>[2x]MLEKVETFDMNRVIDEFDEMTRNAHQVQKQTLKEILLKNQSAIYLQNCGLNGNATDPEEAFKSMVPLVTDVELEPYIKRMVDGDTSPILTGHPVPAISLSSGTSQGRPKFIPFTDELMENTLQLFRTAFAFRNRDFPIDDNGKALQFIFSSKQYISTGGVPVGTATTNVYRNPNFKAGMKSITSPSCSPDEVIFSPDVHQALYCHLLSGILFRDQVQYVFAVFAHGLVHAFRTFEQVWEEIVTDIKDGVLSNRITVPSVRTAMSKLLTPNPELAETIRTKCMSLSNWYGLIPALFPNAKYVYGIMTGSMEPYVPKLRHYAGDLPLVSHDYGSSEGWIAANVTPRLSPEEATFAVIPNLGYFEFLPVSETGEGEEKPVGLTQVKIGEEYEVVITNYAGLYRYRLGDVVKVI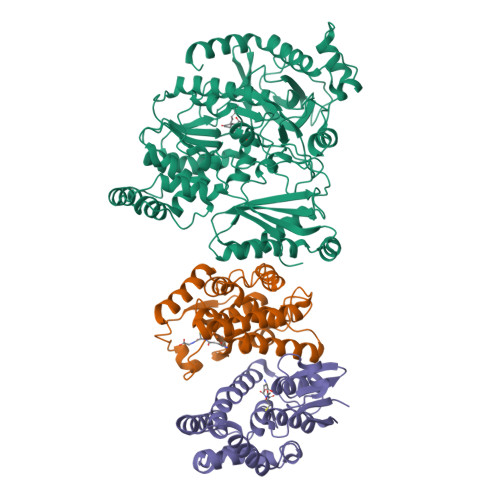GFYNNTPQLKFICRRNLILSINIDKNTERDLQLSVESAAKRLSEEKIEVIDFSSYIDVSTDPGHYAIFWEISGETNEDVLQDCCNCLDRAFIDAGYVSSRKCKTIGALELRVVAKGTFRKIQEHFLGLGSSAGQFKMPRCVKPSNAKVLQILCENVVSSYFSTAF;>[4x]HHHHHHMANLPILLDYWPSMFGMRARVALREKGVEFEYREEDFSNKSPLLLQSNPIHKKIPVLVHNGKPVCESLNVVQYVDEAWPEKNPFFPSDPYGRAQARFWADFVDKKFTDAQFKVWGKKGEEQEAGKKEFIEAVKILESELGDKPYFGGDSFGYVDISLITFSSWFQAYEKFGNFSIESESPKLIAWAKRCMEKESVSKSLPDSEKIVAYAAEYRKNNL> GSHMADKELKFLVV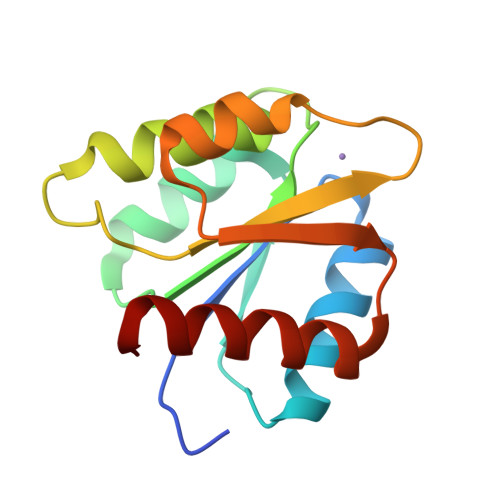DDFSTMRRIVRNLLKELGFNNVEEAEDGVDALNKLQAGGYGFVISDWDMPNMDGLELLKTIRADGAMSALPVLMVTAKAKKENIIAAAQAGASGYVVKPFTAATLEEKLNKIFEKLGM> NGGVGVDVELITSINVENDTFIERNFTPQEIEYCSAQPSVQSSFAGTWSAKEA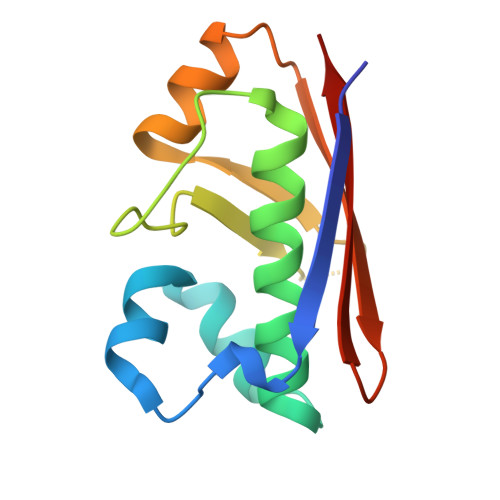VFKSLGVKSLGGGAALKDIEIVRTNKNAPAVELHGNAKKAAEEAGVTDVKVSISHDDLQAVAVAVSTKK>MKSSHHHHHHENLYFQSNAKQALLWRDSETFILTSIELYNWGGFQGYHRAEIDPSGTAVIGPTGSGKTTLVDALMTLLCANPRYNLASTGGHESDRDLVSYVRGVTGPGDGGVEQSHIARQGKTVTAIAATLERDGAQVRLGAVLWFEGTSSSASDLKKLWLLSESPEQTLEHWLSQHHAGGMRALRQMEKDGMGIWPYPSKKAFLARLRDYFEVGENAFTLLNRAAGLKQLNSIDEIFRELVLDDRSAFERAAEVASSFDDLTDIHRELETARKQQRSLQPVADGWERYRALQEQLQDKQALEGILPVWFAEQGYRLWLAETNRLEKEHKQAELDQAQCRSQLEIQKGVVDQHRQRYLRVGGAGIDQLRGRIADWVRECDKRRLKAEQYQRLAKGLGLADELSAAALEENQQQIAARLEILAQQTTDARQKAFDAGLVQQELNGRLQSLQQERAEVERRPGSNLPGHFHAFRGDLAQELGVDESALPFVAELVQVKPEELAWRGAIERAIGSHRLRILVPQGSSQAALRWVNQRHNRLHVRLLEVKEPSSRPVFFDDGFTRKLTFKEHPYREAVKALLADNDRHCVESTEQLRHTPHAMTAQGLMSGKERFFDKQDQKRLDEDWLTGFDNRDRLAFLAEQIREVNEQLVPAKLALDAAQGDVGQLESQASLLQRIEELQFDDIDRPGAERQLQSLRTQLDTLTRPDSNLAVIKAELDQAEALRESLDQQLQRLIEQCVQLKTQFDQAASATRKAYRGAEKGLSDTQRELAQAHFPILSTDDLGDIDELERKHTRELQGQLKTLGEKLGDQKTELAKRMSDALKADTGALAEVGRELVDVPRYLERLRVLTEEALPEKLKRFLEYLNRSSDDGVTQLLSYIDHEVSMIEERLDDLNSTMQRVDFQPGRYLRLVAKKVIHESLRTLQHAQRQLNSARFIDDEGESHYKALQALVGLLKDACEHSRNQGAKALLDPRFRLEFAVSVIDREGNNLIETRTGSQGGSGGEKEIIASYVLTASLSYALCPDGSSRPLFGTIVLDQAFSRSSHAVAGRIIAALREFGLHAVFITPNKEMRLLRHHTRSAVVVHRRGVESSLVSLSWEALDEHHQQRIRAMHEVAH[2x];> MKSSHHHHHHENLYFQ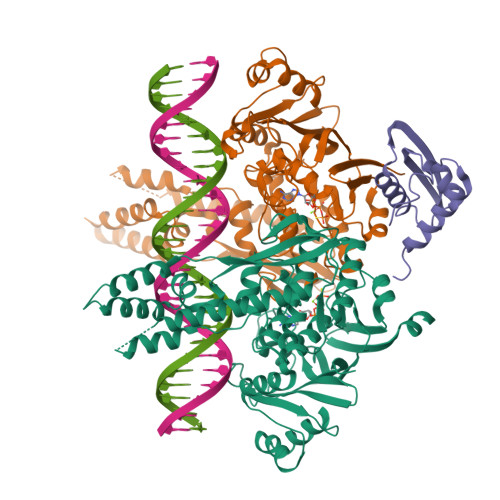SNAEESAQQRSERYVSARSQHPAWLLLASRRAPLVLGCLRTLFERAHDGIPMEDALQALSEMLAAYASQELYEIDPDATHLQAGRELREWIKRRLVVEREGRIYATDALESAIQFVDSLDSRIMTSTASRLSVVQREIENLETGLNPSPTGRIASLRRRIQDLEHELARVEAGHVDVLDEAQAIEGMREVYNLATSLRADFRRVEDSWREADRALRHSIISEQSHRGEIVDRLLDGQDALLNTPEGRVFESFQQQLRQSAELEVMRERLRTILRHPAVPKALNRPQQRELRWLALRLVRESQAVLQARARSERDVRGFMKTGLAAEHHRVGQLLNDFFNLALSVDWQRQSERRKPACLPPVGVAITGVPAIERLRFKTLDDDDAGELDLSLKPAGLEQIDDDFWDAFDGLDREALIHDTLAVLVEQGRPVSLGELASLLPPAHDLETFALWLAMAREAGIEVLTEERQFVELVDEDEQRWGFNLPYVGLDHEALKDIDWEL> XSTSTYALRAGKRDVRREQQEIITRQINTAPYVQDAMMRVVVFAQYPSGRYKAFDY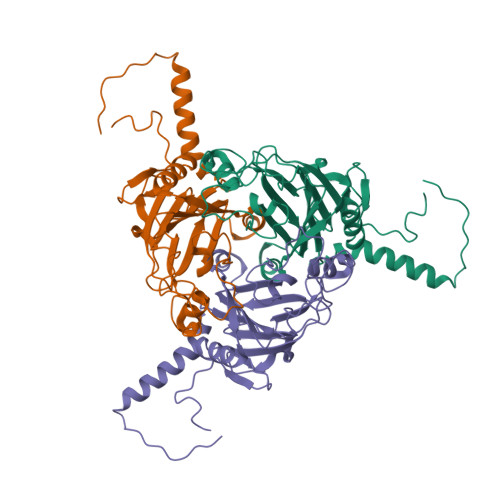VFPDYLKVFLNWRELLEDTTTDYDPRTNTHRLMGQGYRQLIHPNHGSGEEPYDTRYPMGVIVSFNGNIDWTRARVEATNMHGLNNTDWREARAWGPHVICGNQLRKAGHLSRAVYVPLDEHNTVKVLATARQDGALNRFNGPQLAQTLTNNIVCPNVIEFNTESDVIDYAKMAHIAYIDQAGLIVASSDAYISGDSQA> SIVLEPIYWNSSNSKFLPGQGLVLYPQIGDKLDIICPKVDSKTVGQYEYYKVYMVDKDQADRCTIKKENTPLLNCAKPDQDIKFTIKFQEFSPNLWGLEFQKNKDYYI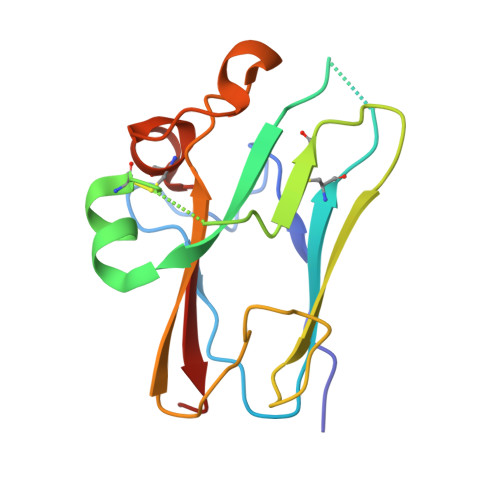ISTSNGSLEGLDNQEGGVCQTRAMKILMKVGQD>MILLDTNVISEPLRPQPNERVVAWLDSLILEDVYLSAITVAEMRLGVALLLNGKKKNVLHERMEQSILPLFAGRILPFDEPVAAIYAQIRSYAKTHGKEIAAADGYIAATAKQHSMTVATRDTGSFFAADVAVFNPWHLEHHH[4x];>[4x]ASVVIRNLSEATHNAIKFRARAAGRSTEAEIRLILDNIAKAQQTVRLGSMLASIGQEIGGVELED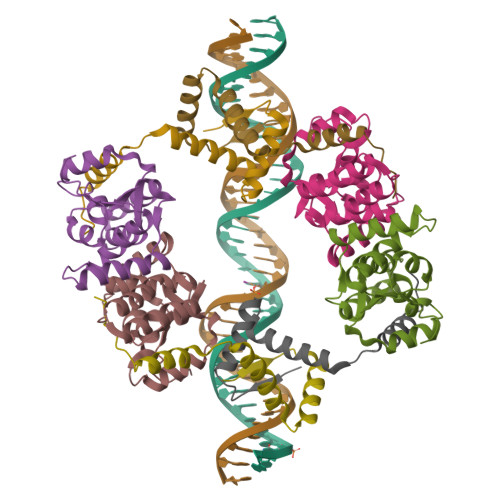VRG> RRRSGSLVYQKRRRRLLPFVSSEDPAQRLKQMGTLASA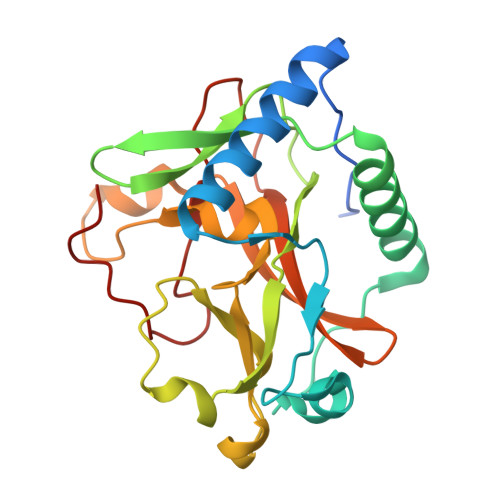LTELQMEFSDDLTYSSGMAPRSANQARFEEGGMQVLTKEDIETLEQCRAMCKRGDCPPLLVVFDSREGFTVEADGQIKDMTFIAEYTGDVDYIRNREHDDCDSMMTLLLAKDPSKSLVICPDKRGNIARFISGINNHTLDGKKKQNCKCVRYSVNGECRVFLVATRDIAKGERLYYDYNGYEHEYPTQHFV>MNLVLMGLPGAGKGTQGERIVEDYGIPHISTGDMFRAAMKEETPLGLEAKSYIDKGELVPDEVTIGIVKERLGKDDCERGFLLDGFPRTVAQAEALEEILEEYGKPIDYVINIEVDKDVLMERLTGRRICSVCGTTYHLVFNPPKTPGICDKDGGELYQRADDNEETVSKRLEVNMKQTQPLLDFYSEKGYLAN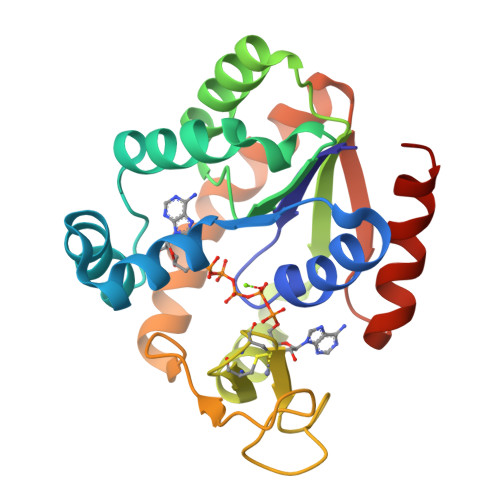VNGQRDIQDVYADVKDLLEGLKK[2x]>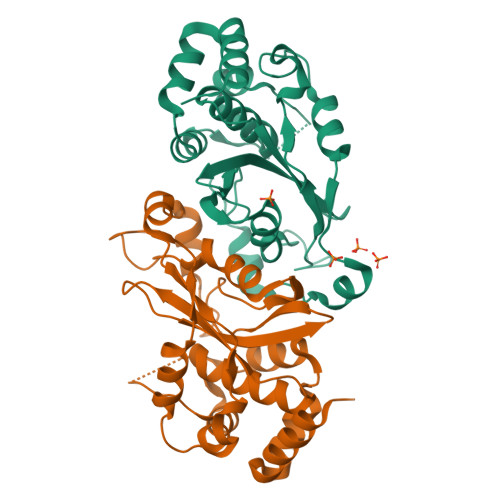[2x]GHMASMTGGQQMGRGSMHYKAQLQKLLTTEEKKILARLSTPQKIQDFLDTIKNKDLAEGEHTMWSPRAVLKHKHAHCMEGAMLAALALAYHGHSPLLMDLQTTDEDEDHVVALFKIDGHWGAISKTNHPVLRYRDPIYKSVRELAMSYFHEYFIWWTKKNGGKKTLRAYSNPFDLTRYKPERWVIATGDLDWLAEALDDSKHFPILNKKMQKQLRPASRIETKAASLSEWPKRKTNS>[3x]MTENAEKFLWGVATSAYQIEGATQEDGRGPSIWDAFAQRPGAIRDGSTGEPACDHYRRYEEDIALMQSLGVRAYRFSVAWPRILPEGRGRINPKGLAFYDRLVDRLLASGITPFLTLYHWDLPLALEERGGWRSRETAFAFAEYA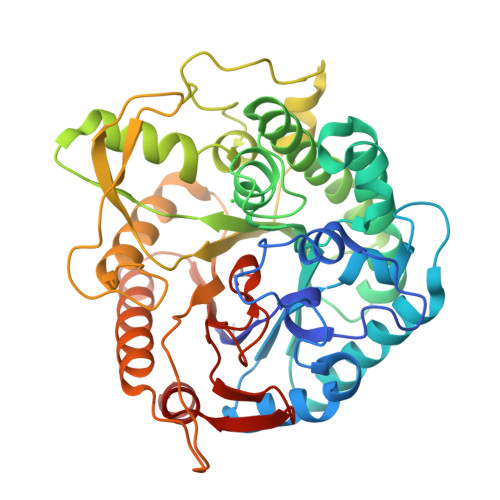EAVARALADRVPFFATLNEPWCSAFLGHWTGEHAPGLRNLEAALRAAHHLLLGHGLAVEALRAAGARRVGIVLNFAPAYGEDPEAVDVADRYHNRFFLDPILGKGYPESPFRDPPPVPILSRDLELVARPLDFLGVNYYAPVRVAPGTGTLPVRYLPPEGPATAMGWEVYPEGLHHLLKRLGREVPWPLYVTENGAAYPDLWTGEAVVEDPERVAYLEAHVEAALRAREEGVDLRGYFVWSLMDNFEWAFGYTRRSGLYYVDFPSQRRIPKRSALWYRERIARAQT>EPGENLKPVDAMQCFDCHTQIEDMHTVGKHATVNCVHCHDATEHVETASSRRMGERPVTRMDLEACATCHTAQFNSFVEVRHESHPRLEKATPTSRSPMFDKLIAGHGFAFEHAEPRSHAFMLVDHFVVDRAYGGRFQFKNWQK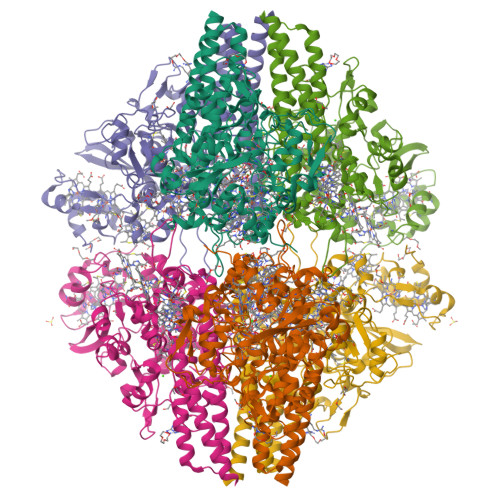VTDGMGAVRGAWTVLTDADPESSDQRRFLSQTATAANPVCLNCKTQDHILDWAYMGDEHEAAKWSRTSEVVEFARDLNHPLNCFMCHDPHSAGPRVVRDGLINAVVDRGLGTYPHDPVKSEQQGMTKVTFQRGREDFRAIGLLDTADSNVMCAQCHVEYNCNPGYQLSDGSRVGMDDRRANHFFWANVFDYKEAAQEIDFFDFRHATTGAALPKLQHPEAETFWGSVHERNGVACADCHMPKVQLENGKVYTSHSQRTPRDMMGQACLNCHAEWTEDQALYAIDYIKNYTHGKIVKSEYWLAKMIDLFPVAKRAGVSEDVLNQARELHYDAHLYWEWWTAENSVGFHNPDQARESLMTSISKSKEAVSLLNDAIDAQVASR[2x]> MGDSILS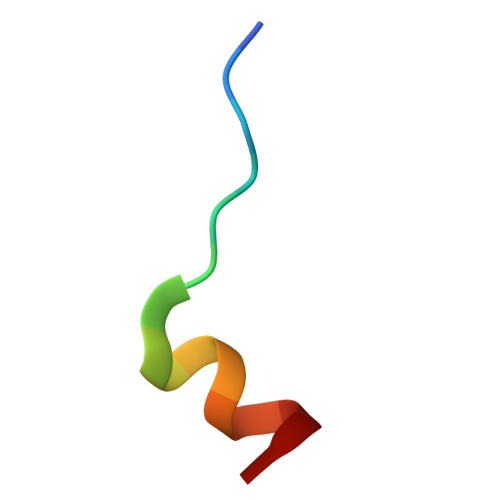QAEIDALLN> MAIYADNSYSIGNTPLVRLKHFGHNGNVVVKIEGRNPSYSVKCRIGANMVWQAEKDGTLTKGKEIVDATSGNTGIALAYVAAARGYKLTLTMPETMSLERKRLLCGLGVNLVLTEGAKGMKGAIAKAEEIVASDPSRYVMLKQFENPANPQIHRETTGPEIWKDTDGKVDVVVAGVGTGGSITGISRAIKLDFGKQITSVAVEPVESPVISQTLAGEEVKPGPHKIQGIGAGFIPKNLDLSIIDRVETVDSDTALATARRLMAEEGILAGISSGAAVAAADRLAKLPEFADKLIVVILPSASE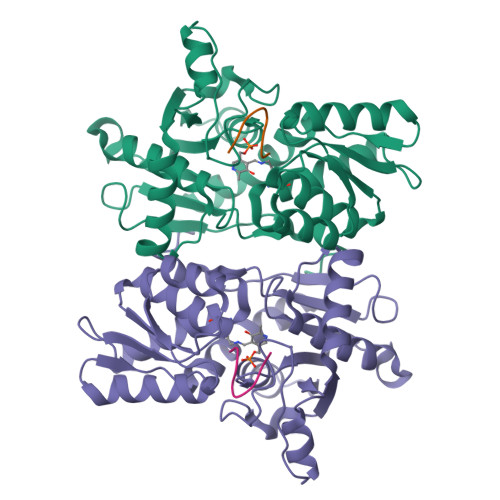RYLSTALFEGIEG;> IGDGYEFT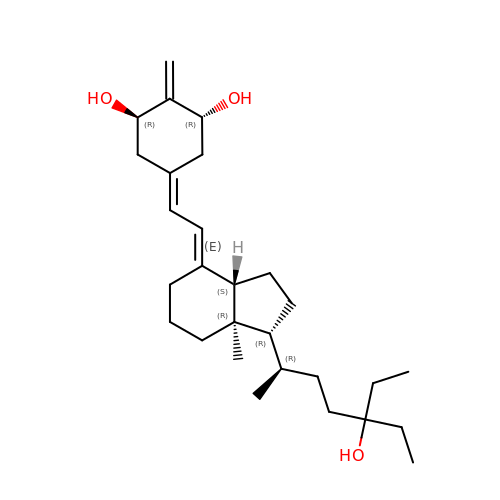(1R,3R,7E,17beta)-17-[(2R)-5-ethyl-5-hydroxyheptan-2-yl]-2-methylidene-9,10-secoestra-5,7-diene-1,3-diol | C28 H46 O3 | CCJKDZZJQKPBID-IHLVXOQFSA-N N-{(3P)-3-[(5P)-5-(2H-tetrazol-5-yl)-2,1-benzoxazol-3-yl]phenyl}cyclopropanecarboxamide | C18 H14 N6 O2 | 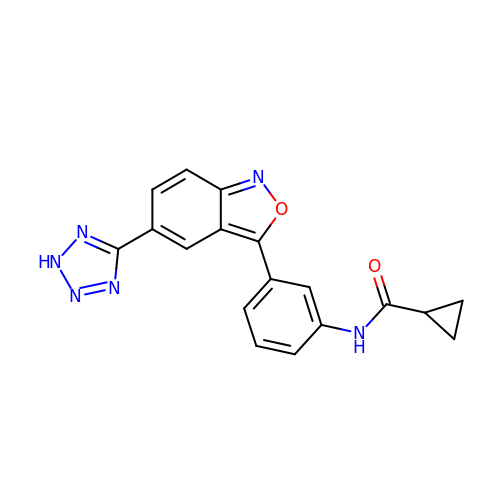ZDYGRDMSDBGSHI-UHFFFAOYSA-N> EK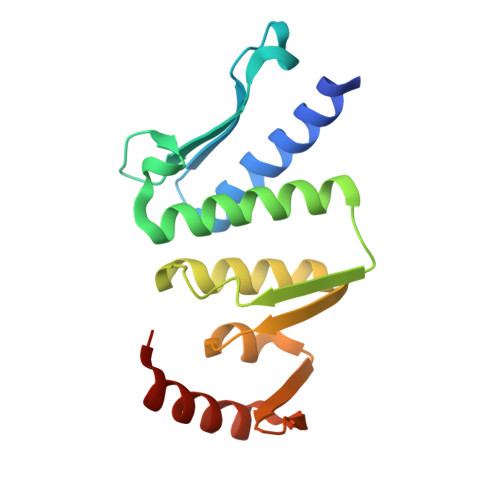EKKNVFMRTFEAISRNFSEIFAKLSPGGSARLILENPEDPFSGGLEIEAKPAGKDVKRIEAMSGGEKALTALAFVFAIQKFKPAPFYLFDEIDAHLDDANVKRVADLIKESSKESQFIVITLRDVMMANADKIIGVSMRDGVSKVVSLSLEKAMKILEEIRKKQGWEHGN Recent work has revealed that ANKS6 interacts with a related protein called ANKS3. Both ANKS6 and ANKS3 have a similar domain structure, with ankyrin repeats at the N-terminus and a SAM domain at the C-terminus. SAM domains consist of approximately 70 amino acids and adopt a globular structure generally containing a core of five α-helices. The protein-protein interactions of SAM domains are typically mediated by two distinct surfaces on the domain, termed the mid-loop (ML) and end-helix (EH) surfaces. Here we define the ANKS6/ANKS3 interaction by discovering that the ANKS6 SAM domain binds to the SAM domain of ANKS3.

To prevent ANKS3-SAM polymerization without destroying ANKS6-SAM binding, we mixed an ML-surface mutant of ANKS3-SAM, I36E, with wild-type ANKS6-SAM. These proteins formed a heterodimer when analyzed by SEC-MALS and yielded crystals suitable for structure determination. The ANKS3-SAM/ANKS6-SAM heterodimer crystallized in space group C2221 with four molecules (2 ANKS3-SAM I36E mutants and 2 ANKS6-SAMs) per asymmetric unit. By solving a crystal structure of the ANKS3-SAM/ANKS6-SAM heterodimer, we observed that the EH-surface of ANKS3-SAM binds the ML-surface of ANKS6-SAM. Additionally, the overall structure of ANKS3-SAM I36E aligns well with ANKS6-SAM (RMSD across backbone atoms is 0.626 Å) with the only obvious difference being a 1.6 Å outward shift of ANKS6-SAM’s helix 3.Similar to the ML-surface of ANKS3-SAM, the ML-surface of ANKS6-SAM contains a shallow hydrophobic patch (residues V30, A34, L38, L46) flanked by negatively charged residues (E29, D31, E33, D42, E45). Many of these charged residues form salt bridges with ANKS3-SAM (ANKS6 E29 + ANKS3 K22, ANKS6 D31 + ANKS3 K58, ANKS6 D42 + ANKS3 R57). The decreased steric bulk of Ala compared to Ile allows helix 3 of ANKS6-SAM’s ML-surface to approach the EH-surface of ANKS3-SAM more closely, resulting in the burial of additional surface area and the formation of more salt bridges and hydrogen bonds, which may explain the higher affinity of the ANKS3-SAM/ANKS6-SAM interface. The ANKS6-SAM structure also shows that the EH-surface is lacking a large hydrophobic residue flanked by positively charged residues, thereby showing that ANKS6-SAM cannot polymerize because its EH-surface is incompatible with binding its ML-surface. R823 (R54 in the crystal structure numbering) forms salt bridges with D51 of helix 5 and D40 of helix 4, and forms hydrogen bonds with the backbone carbonyls of I48 and K49 which both lie on a loop between helices 4 and 5. Through these interactions, R54 is involved in stapling helices 4 and 5 and in maintaining the overall fold in this segment of the domain.

>SRAPYSGPQDLAALLEQIGCLKYLQVFEEQDVDLREFLTLTESDLKEIGITLFGPKRKMTSAIARWHSSAR[2x];>[2x]STITDEDELTGILKKLSLEKYQPIFEEQEVDMEAFLTLTDGDLKELGIKTDGSRQQILAAISELNAGKGRE3-[[4-[(3,4-dichlorophenyl)methyl]piperidin-4-yl]methoxy]pyridine | C18 H20 Cl2 N2 O | 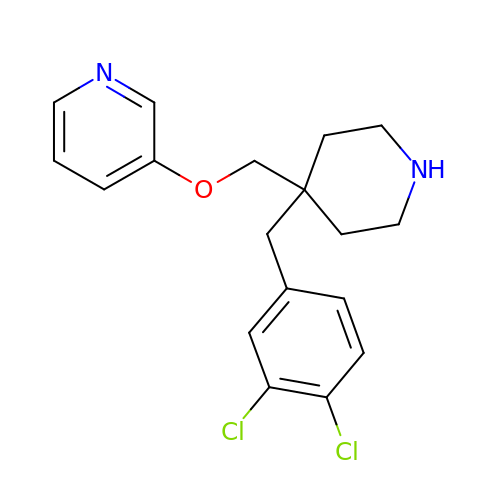DFIMBYYXCVFOEJ-UHFFFAOYSA-N>GASMTIEDEYSGPKLEDGKVTISFMKELMQWYKDQKKLHRKCAYQILVQVKEVLSKLSTLVETTLKETEKITVCGDTHGQFYDLLNIFELNGLPSETNPYIFNGDFVDRGSFSVEVILTLFGFKLLYPDHFHLLRGNHETDNMNQIYGFEGEVKAKYTAQMYELFSEVFEWLPLAQCINGKVLIMHGGLFSEDGVTLDDIRKIERNRQPPDSGPMCDLLWSDPQPQNGRSISKRGVSCQFGPDVTK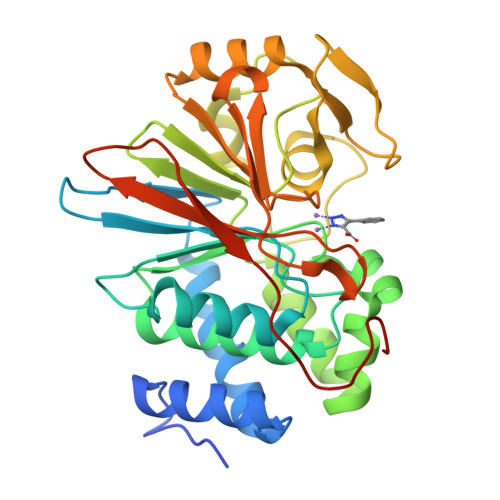AFLEENNLDYIIRSHEVKAEGYEVAHGGRCVTVFSAPNYCDQMGNKASYIHLQGSDLRPQFHQFTAVPHPNVKPMAYANTLLQLGMM[4x]2-AMINO-4-(2-AMINO-ETHOXY)-BUTYRIC ACID | C6 H14 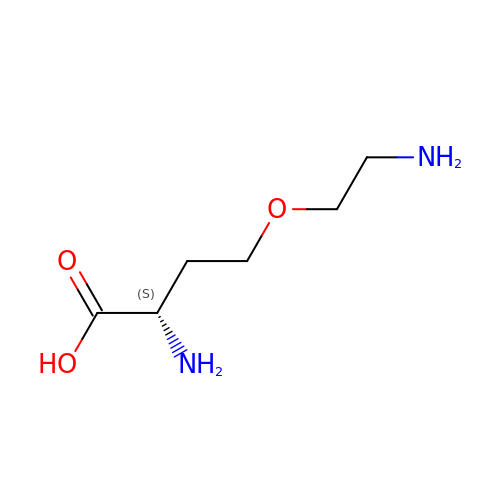N2 O3 | FDDYPVBIHWFLOI-YFKPBYRVSA-N> GPIPTAPRENSLMFLSTLPDDTVPAYGNVRTPPVNYLPGEITDLLQLARIPTLMAFERVPEPVPASDTYVPYVAVPTQFD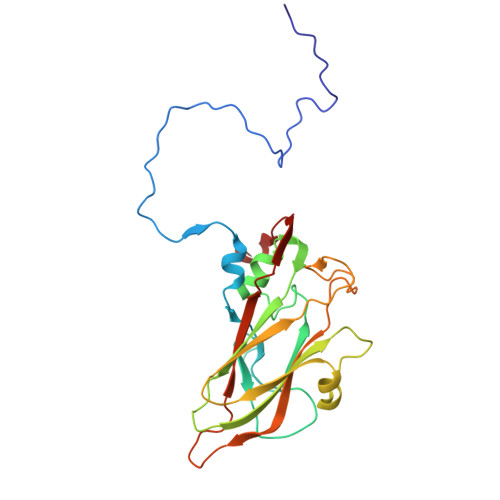DRPLISFPITLSDPVYQNTLVGAISSNFANYRGCIQITLTFCGPMMARGKFLLSYSPPNGTQPQTLSEAMQCTYSIWDIGLNSSWTFVVPYISPSDYRETRAITNSVYSADGWFSLHKLTKITLPPDCPQSPCILFFASAGEDYTLRLPVDCNPSYVFH>MGGSHHHHHHGENLYFQSVDDLTVEPNLHSLITSTTHKWIFVGGKGGVGKTTSSCSIAIQMALSQPNKQFLLISTDPAHNLSDAFGEKFGKDARKVTGMNNLSCMEIDPSAALKDMNDMAVSRANNNGSDGQGDDLGSLLQGGALADLTGSIPGIDEALSFMEVMKHIKRQEQGEGETFDTVIFDTAPTGHTLRFLQLPNTLSKLLEKFGEITNKLGPMLNSFMGAGNVDISGKLNELKANVETIRQQFTDPDLTTFVCVCISEFLSLYETERLIQELISYDMDVNSIIVNQLLFAENDQEHNCKRCQARWKMQKKYLDQIDELYEDFHVVKMPLCAGEIRGLNNLTKFSQFLNKEYNPITDGKVIYELEDKE[8x];>MGAKLAKTLQRFENKIKAGDYYEAHQTLRTIANRYVRSKSYEHAIELISQGALSFLKAKQGGSGTDLIFYLLEVYDLAEVKVDDISVARLVRLIAELDPSEPNLKDVITGMNNWSIKFSEYKFGDPYLHNTIGSKLLEGDFVYEAERYFMLGTHDSMIKYVDLLWDWLCQVDDIEDSTVAEFFSRLVFNYLFISNISFAHESKDIFLERFIEKFHPKYEKIDKNGYEIVFFEDYSDLNFLQLLLITCQTADASYFLNLKNHYLDFSQAYKSELEFLGQEYFNIVAPKQTNFLQDMMSGFLGGSGEN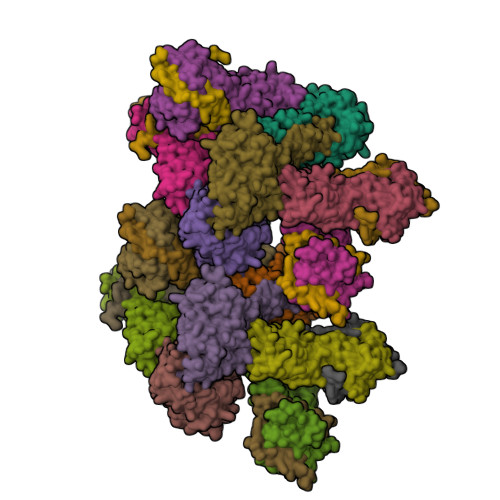LYFQSLEHHHHHH[8x];>MSTSASGPEHEFVSKFLTLATLTEPKLPKSYTKPLKDVTNLGVPLPTLKYKYKQNR[8x]>GPLGSPEFGYWITCCPTCDVDINTWVPFYSTELNKPAMIYCSHGDGHWVHAQCMDLEERT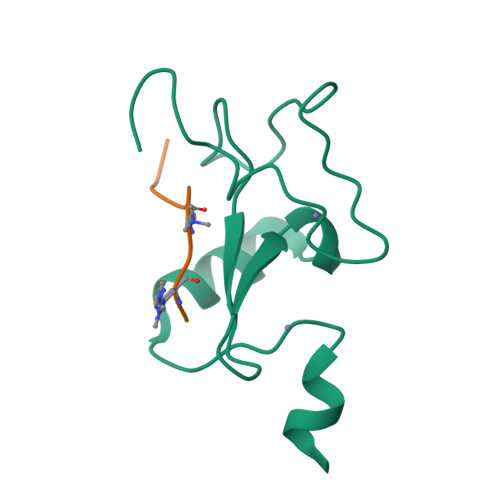LIHLSEGSNKYYCNEHVQIARA[2x];>[2x]ARTKQTARA>[2x]SAVPSD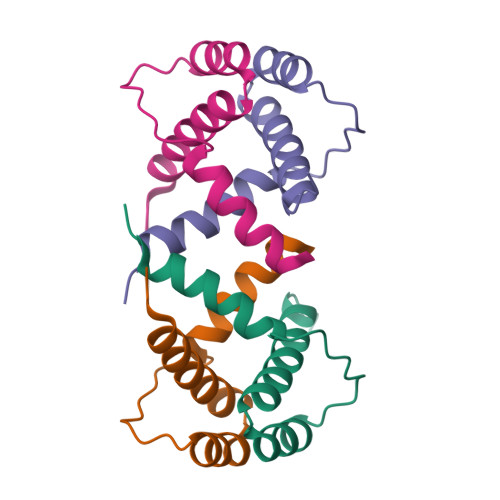SQAREKLALYVYEYLLHVGAQKSAQTFLSEIRWEKNITLGEPPGFLHSWWCVFWDLYCAAPE>MLVATLTLVALSAVFTNVYGSDQYTILDVYKASNVSVEDYKDLLKDLDVVHSFKVLGSSRVIFVVKMREDSYEKLSKINLPGDVYSIPAGDLSDKMQSVGVEWKRWDDLPDANLTLFERTLELKGEPLEGLASHMKAFGEKVSHVMELYPNKGFYLLGRTPPKAFVIVSLPFRCRQVRYGSDFALNYLNGPGDSSTKVEFVAKA[2x];>[2x]MYALAIALLAFSTFVSNAFANKEYLLLDIRDATTSEIISALRDVEIELKVKAKGIARHLIVVKQNDANLQKLGEIDIPGRSCSTPVEDLDNLMEDIGISWPRNELTNVNVTLFERTLDLKDKTMEQFWSEAKAYGQLVKPVLSSFTYRAFKANGAYPPKVYFFVNLPRENLNDASSKGIDIFGGPGKARTTVQYVTKLS;>[2x]MFVATSLLLAIATLVVRASPHNYLIMDIEPPKSVSERDILNLLSPLQVKHSFRVTGSTRLLIVIRLDAQSYEKLDEITVPGKVEVIPAVNMADTMERCGVSWPRVELTDDNVTLFESESTLTDVTKEQLKAMLIGYGEHMSGLLQAHRFEYYQAAGATPHRHFVFVNSVPDEI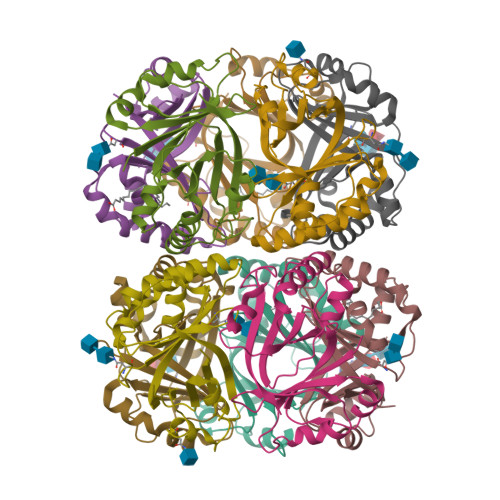EVFGREGVDIWGGPGEFVVKPQYVTRI;>[2x]MTAILALLLAMSILLPSGAVEDVQDLVFAEWDKGSSHEHACSALRNSSVIEKGLTVKEVGTSKFAAVLSEPILARLKFHGLVEAVPVVEVGTVMKRLNVSIPPAQDISDNNLTLIKMSPKLKGQTLQQIDAELRYLGEYMNTVLQKCSHRVYISKGTFPPKIYVFLNMPLDQIRQFYPSLDIFGGPSSTKNEISYVQILILRN;>[2x]MAEHRIPVLLLLVVVAASSLAQQIPLQKHYIIYEVRNIEKTPEEVKEEMKDTDILYSFKALGAPSYHIVVEVNPRNMRKLEEVELKGKIRMVPVVNMVDVAETLGVSWPRSGARLLDVNLTLIERTLNQEGLTSQESEAHLKGFMEELKDRLQQYNYQAFFTIGASPPKMYIYINIPYEEVDKFACIGINQFGGPAAVNTTVSFISSFPK> GMSEKPKVYQGVRVKITVKELLQQRRAHQAA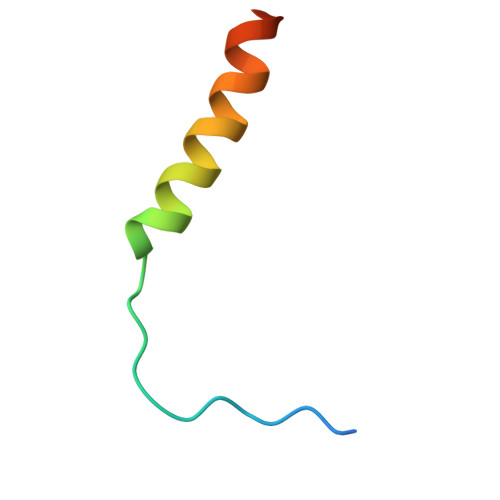SGGTRSGG> PTGKLWRPVGTSVATIDSLAIVSDRFGQYSFVNEGMRETFSKALFDINMWQPLFQATKTGCGPIVLSSFTTTTSGYVGATAGDALDNPVTNGVFISTVQIMNLQRTIAARMRDVALWQKHLDTAMTMLTPDISAGSASCNWKSLLAFAKDILPLDNLCLTYPNEFYNVAIHRYPALKPGNPDTKLPDAQAHPLGEVAGAFNAATSEVGSLVGSSSTLSQAISTMAGKDLDLIEADTPLPVSVFTPSLAPRSYRPAFIKPEDAKWIAEFNNSSLIRKTLTYSGATYTVQLGPGPTRVIDMNAMIDSVLTLDVSGTILPYDTNPDLSTSVPAFVLIQTSVPIQQVTTAANITAITVVSAAGASAINLAINVRGQPRFNMLHLQATFERETITGIPYIYGLGTFLIPSPTSSSNFSNPTLMDGLLTVTPVLLRETTYKGEVVDAIVPATVMANQTSEEVASALANDAIVLVSNHLNKLANVVGDAIPVASRTDDSATSAIVSRLAVQHKLSQVGQASPTPPDYPLLWRRAKRAASMFVSNPSLALQVGIPVLTQSGMLSALTSGVGTALRTGSLGKGVTDASEKLRARQSLTVAKQAFFDQIGSLWP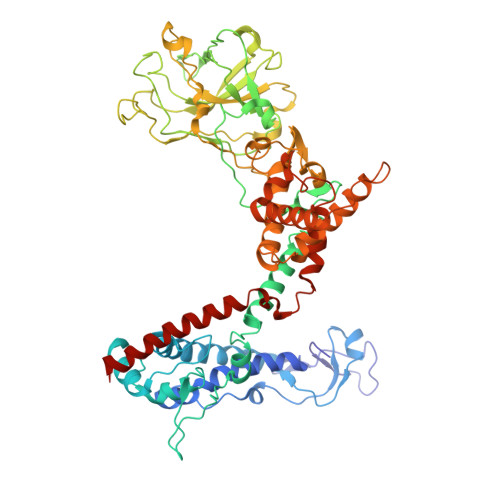GK(3S)-5-(4'-ACETYLBIPHENYL-4-YL)-3-HYDROXYPENTANOIC ACID | C19 H20 O4 | 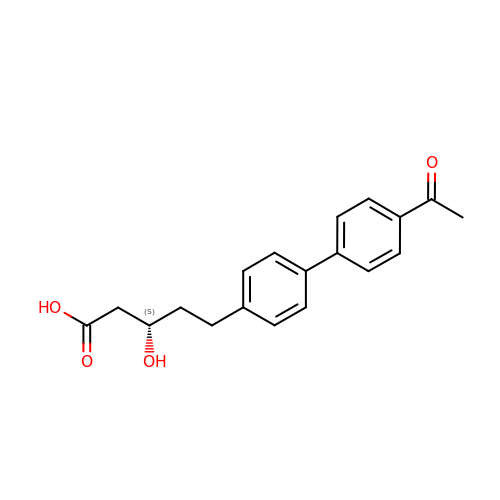QSVVRYPBRVSBDL-SFHVURJKSA-N> MKTSDANETEDHLESLICKVGEKSACSLESNLEGLAGVLEADLPNYKSKILRLLCTVARLLPEKLTIYTTLVGLLNARNYNFGGEFVEAMIRQLKESLKANNYNEAVYLVRFLSDLVNCHVIAAPSMVAMFENFVSVTQEEDVPQVRRDWYVYAFLSSLPWVGKELYEKKDAEMDRIFANTESYLKRRQKTHVPMLQVWTADKPHPQEEYLDCLWAQIQKLKKDRWQERHILRPYLAFDSILCEALQHNLPPFTPPPHTEDSVYPMPRVIFRMFDYTDDPEGPVMPGSHSVERFVIEENLHCIIKSHWKERKTCAAQLVSYPGKNKIPLNYHIVEVIFAELFQLPAPPHIDVMYTTLLIELCKLQPGSLPQVLAQATEMLYMRLDTMNTTCVDRFINWFSHHLSNFQFRWSWEDWSDCLSQDPESPKPKFVREVLEKCMRLSYHQRILDIVPPTFSALCPANPTCIYKYGDESSNSLPGHSVALCLAVAFKSKATNDEIFSILKDVPNPNQDDDDDEGFSFNPLKIEVFVQTLLHLAAKSFSHSFSALAKFHEVFKTLAESDEGKLHVLRVMFEVWRNHPQMIAVLVDKMIRTQIVDCAAVANWIFSSELSRDFTRLFVWEILHSTIRKMNKHVLKIQKELEEAKEKLARQHKRRSDD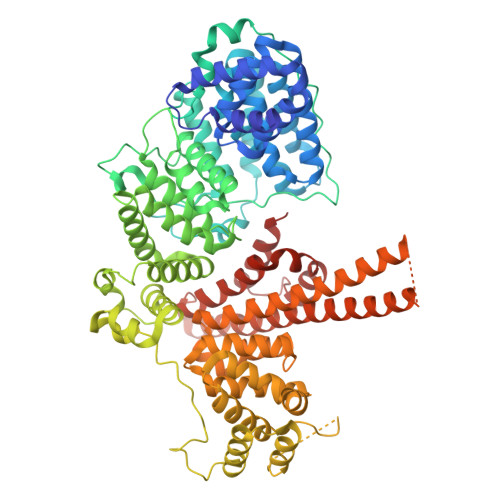DDRSSDRKDGVLEEQIERLQEKVESAQSEQKNLFLVIFQRFIMILTEHLVRCETDGTSVLTPWYKNCIERLQQIFLQHHQIIQQYMVTLENLLFTAELDPHILAVFQQFCALQA>[2x]MSAKSRTIGIIGAPFSKGQPRGGVEEGP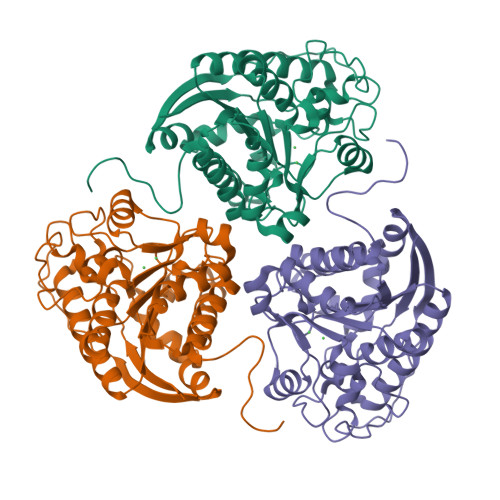TVLRKAGLLEKLKEQECDVKDYGDLPFADIPNDSPFQIVKNPRSVGKASEQLAGKVAEVKKNGRISLVLGGDHSLAIGSISGHARVHPDLGVIWVDAHTDINTPLTTTSGNLHGQPVSFLLKELKGKIPDVPGFSWVTPCISAKDIVYIGLRDVDPGEHYILKTLGIKYFSMTEVDRLGIGKVMEETLSYLLGRKKRPIHLSFDVDGLDPSFTPATGTPVVGGLTYREGLYITEEIYKTGLLSGLDIMEVNPSLGKTPEEVTRTVNTAVAITLACFGLAREGNHKPIDYLNPPK>[2x]MHHHHHHENLYFQGADESFNLWQECATRCTLDLAQGVRASQLDVASLLGEQAGSGVLHYSMVLEEGGDSLKLALGNALTLRTDGTTITLTSATAGKGPRTYSYTRQGRGNWSLHWLVPVGDDAPASIKVFFHELDAGSEVSHISPIYSIEVSDDLLRTMASNSTLFVRHVENNEINRSLTLSAAGVGFVAAPTQHSRQKRWSEWHTGKVLCLLDPLDAVYNYLSQRTCNLGDTWEGKVYRVLAGTPASHDTHIVPTAISHRLHFAKGDGLAALTTHQVCAIPLESLARSRQPRGWEELSQCGYPVHNLVT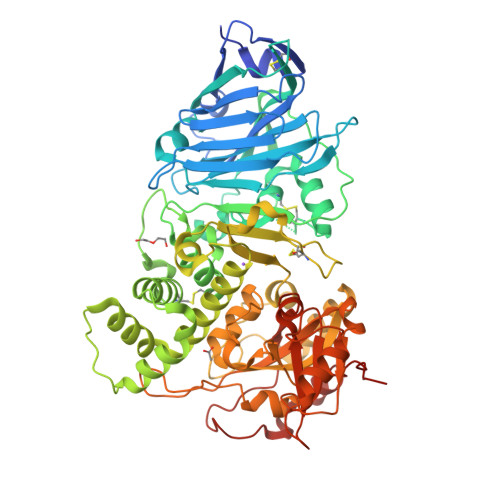LYLLTRLPWSQLDTVITQALANTTPEDGSTPRGQLAQAIRENPAQARLALSMAAAQSDAFSHQQAGNSQEQAASADVVNLTCPAADLNCLAPADSADALQERDYPNGASFLGDGDEVSFSTAGTRNWSVTRLEQAHRQLLARGYLFVGYHGTFLEAAHSIVFEGVHERDQSSIAPWQGFYVAGDPALAYGYAQDQEADARGRIRNGVLLRVYVPRAALPRLFATQQTLAAPGAVDEIGRLIGHPLPLQLEAITGPEEEGGRLATILGWRLAEQAVVIPSTIPTDPRNVGGDLDPASVPQEESAISTLPDYTTQPRDEL>[2x]MGVVEEAHNVKVIGSGEATIVLGHGFGTDQSVWKHLVPHLVDDYRVVLYDNMGAGTTNPDYFDFDRYSNLEGYSFDLIAILEDLKIESCIFVGHSVSAMIGVLASLNRPDLFSKIVMISASPRYVNDVDYQGGFEQEDLNQLFEAIRSNYKAWCLGFAPLAVGGD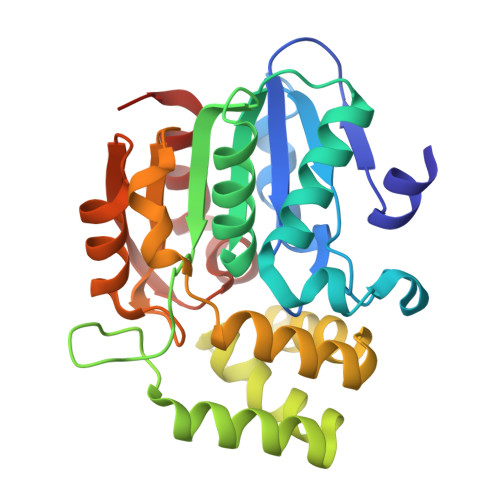MDSIAVQEFSRTLFNMRPDIALSVGQTIFQSDMRQILPFVTVPCHILQSVKDLAVPVVVSEYLHANLGCESVVEVIPSDGHLPQLSSPDSVIPVILRHIRNDIAM>SNAMNIQALLSEKVSQALIAAGAPADCEPQVRQSAKVQFGDYQANGVMAVAKKLGMAPRQLAEQVLSHLDLNGIANKVEIA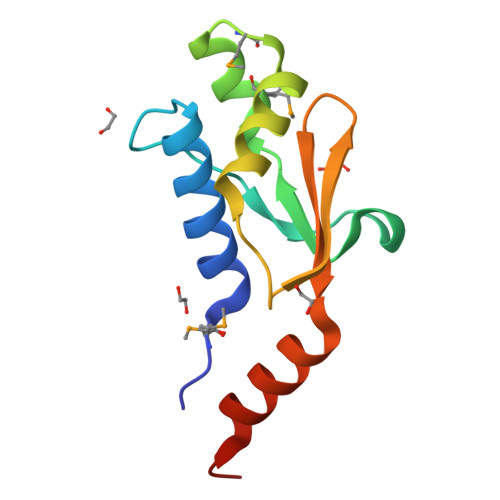GPGFINIFLDPAFLADNVNRALQSERLG[4x]>SGNNFEYTLEASKSLRQKPGDSTMTYLNKGQFYPITLKEVSSSEGIHHPISKVRSVIMVVFAEDKSREDQLRHWKYWHSRQHTAKQRCIDIADYKESFNTISNVEEIAYNAISFTWDINDEAKVFISVNCLSTDFSSQKGVKGLPLNIQIDTYSYNNRSNKPVHRAYCQIKVFCDKGAERKIRDEERKQSKRKVSDVKVPLLPSHKRMDITVFKPFIDLDT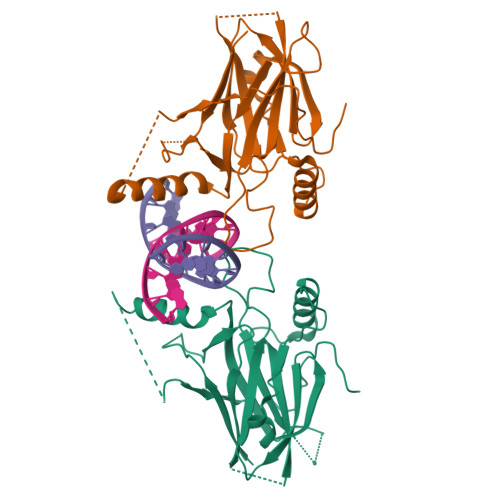QPVLFIPDVHFANLQRG[2x]> GPLGSMSFLKTVPEELTAAAAQLGTIGAAMAAQNAAAAAPTTAIAPAALDEVSALQAALFTAYGTFYQQVSAEAQAMHDMFVNTLGISAGTYGVTESLNSSAAA;> HHHHHHHMMDFGALPPEINSARMYAGAGAGPMMAAGAAWNGLAAELGTTAASYESVITRLTTESWMGPASMAMVAAAQPYLAWLTYTAEAAAHAGSQAMASAAAYEAAYAMTVPPEVVAANRALLAALVATNVLGINTPAIMATEALYAEMWAQDALAMYGYAAASG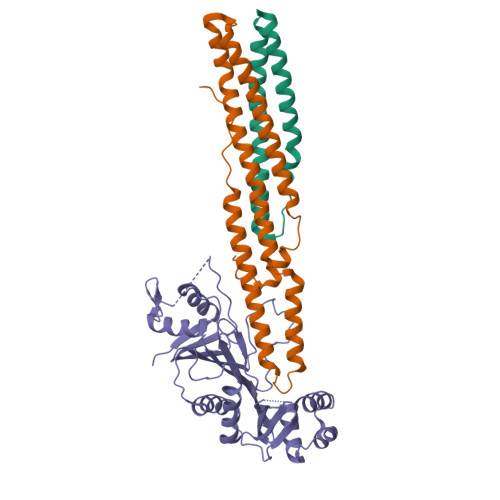AAGMLQPLSPPSQTTNPGGLAAQSAAVGSAAATAA;> HHHHHHHMMDQQSTRTDITVNVDGFWMLQALLDIRHVAPELRCRPYVSTDSNDWLNEHPGMAVMREQGIVVNDAVNEQVAARMKVLAAPDLEVVALLSRGKLLYGVIDDENQPPGSRDIPDNEFRVVLARRGQHWVSAVRVGNDITVDDVTVSDSASIAALVMDGLESIHHADPAAINAVNVPMEEMLEATKSWQESGFNVFSGGDLRRMGISAATVAALGQALSDPAAEVAVYARQYRDDAKGPSASVLSLKDGSGGRIALYQQARTAGSGEAWLAICPATPQLVQVGVKTVLDTLPYGEWKTHSRV>MDQKQFEKIRAVFDRSGVALTLVDMSLPEQPLVLANPPFLRMTGYTEGQILGFNCRFLQRGDENAQARADIRDALKLGRELQVVLRNYRANDEPFDNLLFLHPVGGRPGA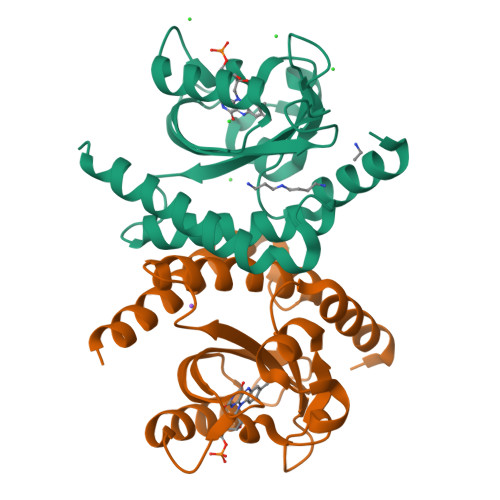PDYFLGSQFELGRSGNSEEAAAAGHAGALTGELARIGTVAARLEMDSRRHLAQAAAALVRAWERRG[6x]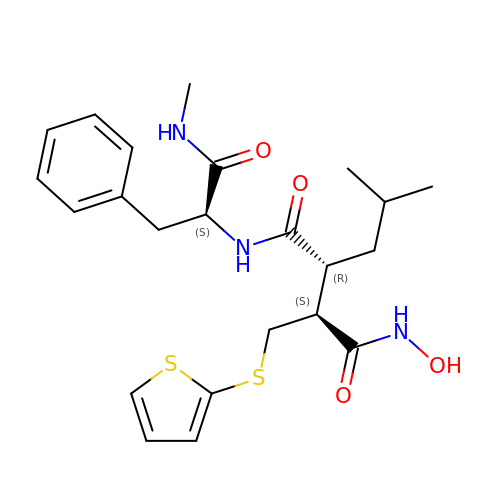4-(N-HYDROXYAMINO)-2R-ISOBUTYL-2S-(2-THIENYLTHIOMETHYL)SUCCINYL-L-PHENYLALANINE-N-METHYLAMIDE | C23 H31 N3 O4 S2 | XFILPEOLDIKJHX-QYZOEREBSA-N> MEDLIDGIIFAANYLGSTQLLSDKTPSKNVRMMQAQEAVSRI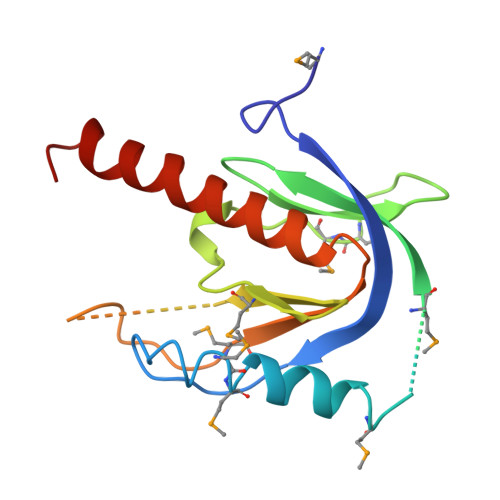KMAQKLAKSRKKAPEGESQPMTEVDLFILTQRIKVLNADTQETMMDHPLRTISYIADIGNIVVLMARRRIPRSNSQENVEASHPSQDGKRQYKMICHVFESEDAQLIAQSIGQAFSVAYQEFLRANGINP>[4x]MAKVSLEKDKIKFLLVEGVHQKALESLRAAGYTNIEFHKGALDDEQLKESIRDAHFIGLRSRTHLTEDVINAAEKLVAIGAFAIGTNQVDLDAAAKRGIPVFNAPFSNTRSVAELVIGELLLLLRGVPEAN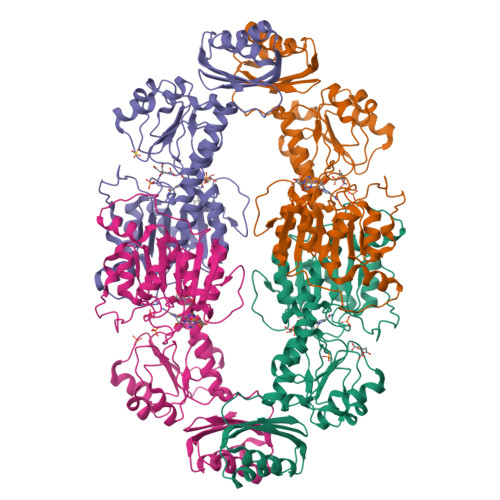AKAHRGVWNKLAAGSFEARGKKLGIIGYGHIGTQLGILAESLGMYVYFYDIENKLPLGNATQVQHLSDLLNMSDVVSLHVPENPSTKNMMGAKEISLMKPGSLLINASRGTVVDIPALADALASKHLAGAAIDVFPTEPATNSDPFTSPLAEFDNVLLTPHIGGSTQEAQENIGLEVAGKLIKYSDNGSTLSAVNFPEVSLPLHVGRRLMHIHENRPGVLTALNKIFAEQGVNIAAQYLQTSAQMGYVVIDIEADEDVAEKALQAMKAIPGTIRARLLY> SNAEASRVYEIIVESVVNEVREDFENAGIDEQTLQDLKNIWQKKLTET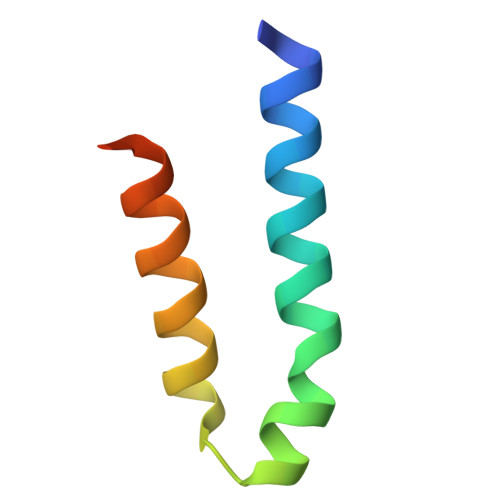KVTTF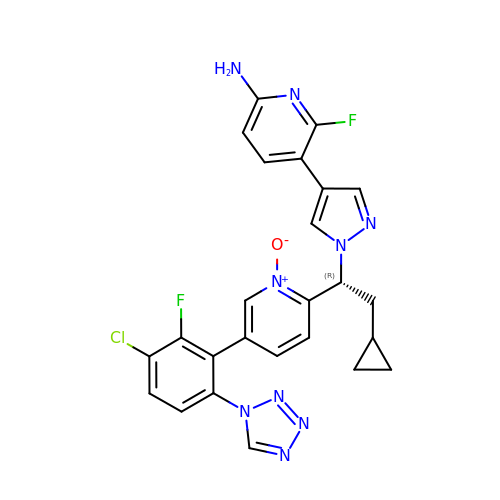5-[1-[(1~{R})-1-[5-[3-chloranyl-2-fluoranyl-6-(1,2,3,4-tetrazol-1-yl)phenyl]-1-oxidanyl-pyridin-2-yl]-2-cyclopropyl-ethyl]pyrazol-4-yl]-6-fluoranyl-pyridin-2-amine | C25 H20 Cl F2 N9 O | QBLULMRFSPWMPT-OAQYLSRUSA-N> MVPISPIETVPVKLKPGMDGPKVKQWPLTEEKIKALVEICTEMEKEGKISKIGPENPYNTPVFAIKKKDSTKWRKLVDFRE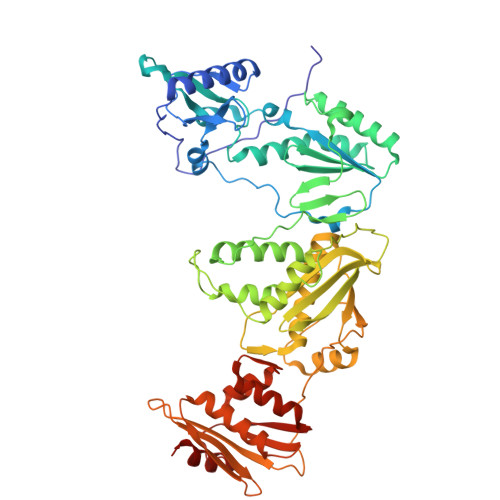LNKRTQDFWEVQLGIPHPAGLKKKKSVTVLDVGDAYFSVPLDEDFRKYTAFTIPSINNETPGIRYQYNVLPQGWKGSPAIFQSSMTKILEPFKKQNPDIVIYQYMDDLYVGSDLEIGQHRTKIEELRQHLLRWGLTTPDKKHQKEPPFLWMGYELHPDKWTVQPIVLPEKDSWTVNDIQKLVGKLNWASQIYPGIKVRQLSKLLRGTKALTEVIPLTEEAELELAENREILKEPVHGVYYDPSKDLIAEIQKQGQGQWTYQIYQEPFKNLKTGKYARMRGAHTNDVKQLTEAVQKITTESIVIWGKTPKFKLPIQKETWETWWTEYWQATWIPEWEFVNTPPLVKLWYQLEKEPIVGAETFYVDGAANRETKLGKAGYVTNKGRQKVVPLTNTTNQKTELQAIYLALQDSGLEVNIVTDSQYALGIIQAQPDKSESELVNQIIEQLIKKEKVYLAWVPAHKGIGGNEQVDKLVSAG>[6x]MDAAIRGNDVIFVLKTIGVPSACRQNEDPRFVEAFKCDELERYIDNNPECTLFESLRDEEAYSIVRIFMDVDLDACLDEIDYLTA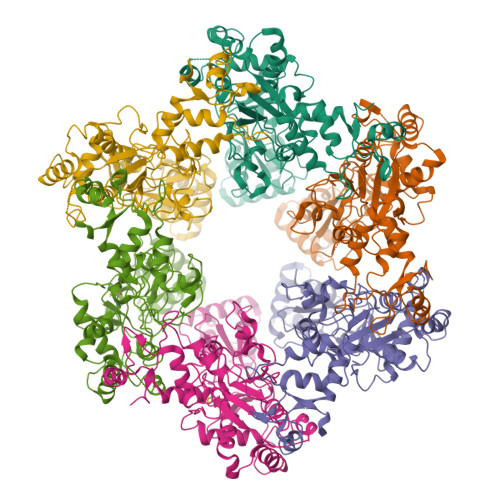IQDFIIEVSNCVARFAFTECGAIHENVIKSMRSNFSLTKSTNRDKTSFHIIFLDTYTTMDTLIAMKRTLLELSRSSENPLTRSIDTAVYRRKTTLRVVGTRKNPNCDTIHVMQPPHDNIEDYLFTYVDMNNNSYYFSLQRRLEDLVPDKLWEPGFISFEDAIKRVSKIFINSIINFNDLDENNFTTVPLVIDYVTPCALCKKRSHKHPHQLSLENGAIRIYKTGNPHSCKVKIVPLDGNKLFNIAQRILDTNSVLLTERGDHIVWINNSWKFNSEEPLITKLILSIRHQLPKEYSSELLCPRKRKTVEANIRDMLVDSVETDTYPDKLPFKNGVLDLVDGMFYSGDDAKKYTCTVSTGFKFDDTKFVEDSPEMEELMNIINDIQPLTDENKKNRELYEKTLSSCLCGATKGCLTFFFGETATGKSTTKRLLKSAIGDLFVETGQTILTDVLDKGPNPFIANMHLKRSVFCSELPDFACSGSKKIRSDNIKKLTEPCVIGRPCFSNKINNRNHATIIIDTNYKPVFDRIDNALMRRIAVVRFRTHFSQPSGREAAENNDAYDKVKLLDEGLDGKIQNNRYRFAFLYLLVKWYKKYHIPIMKLYPTPEEIPDFAFYLKIGTLLVSSSVKHIPLMTDLSKKGYILYDNVVTLPLTTFQQKISKYFNSRLFGHDIESFINRHKKFANVSDEYLQYIFIEDISSP> MRKFCHFMANCWNSARSHATYGAVPLTHSQVTSVYATDGGKVDELGLLELVEERIFSWKLNKWEMRIPPNLPNDQKELIRQEQENLKQILSEWRKCFGALNADILQISSLTGVPKDVVREKNRTWLQEEVAKLRWMGEVNKAALLRDAFMRL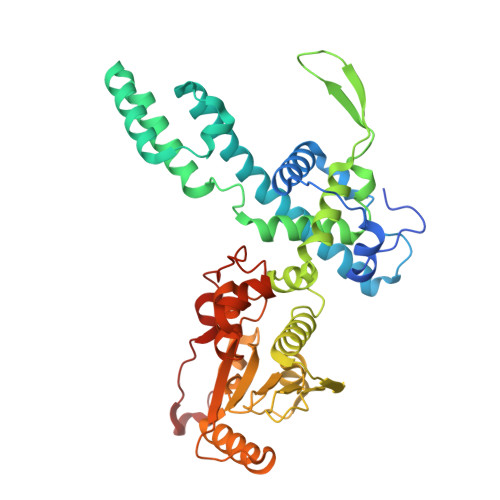EAFGSRDFMFMERLCCIYGLARQGTFDEAFTNYITEDPVTNDIFVDERNPFKELVAHIVRNYSQIDIIYDFLGFNYSEGYRSSLRRYMEYLQCKTAENVRASGRLVTGDKGEHNILFDYCVSRESLVSGDSCQGIIDFLYINGNDVTLIIIASDNPWLRNRQLPHRRQMEGIARRVCFVLGIPPSEVRIRNLLLPPTYLDKGSIVRLNDIVFRLSNEQSNLLIPWLTNYNKELDPKDVDYTALAKTTNEEEWLTL>[2x]MAETPNSDMSGATGGRSKRPKSNQDWWPSKLNLEILDQNARDVGPVEDDFDYAEEFQKLDLEAVKSDLEEL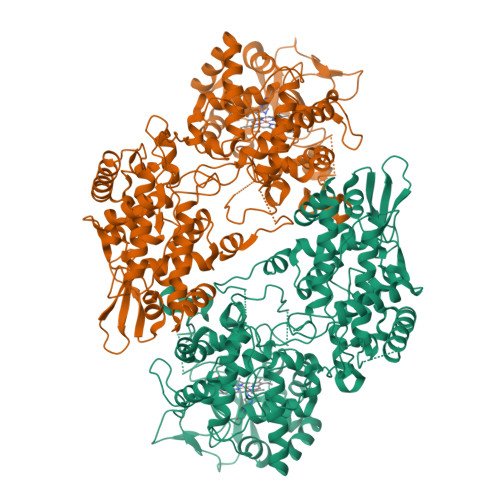MTSSQDWWPADYGHYGPLFIRMAWHSAGTYRTADGRGGAAGGRQRFAPINSWPDNANLDKARRLLLPIKQKYGQKISWADLMILAGNVAIESMGFKTFGYAGGREDAFEEDKAVNWGPEDEFETQERFDEPGEIQEGLGASVMGLIYVNPEGPDGNPDPEASAKNIRQTFDRAAMNDKETAALIAGGHTFGKVHGADDPEENLGPEPEAAPIEQQGLGWQNKNGNSKGGEMITSGIEGPWTQSPTEWDMGYINNLLDYEWEPEKGPGGAWQWAPKSEELKNSVPDAHDPDEKQTPMMLTTDIALKRDPDYREVMETFQENPMEFGMNFAKAWYKLTHRDMGPPERFLGPEVPDEEMIWQDPLPDADYDLIGDEEIAELKEEILDSDLSVSQLVKTAWASASTYRDSDKRGGANGARLRLEPQKNWEVNEPEQLETVLGTLENIQTEFNDSRSDGTQVSLADLIVLGGNAAVEQAAANAGYDVEIPFEPGRVDAGPEHTDAPSFDALKPKVDGVRNYIQDDITRPAEEVLVDNADLLNLTASELTALIGGMRSIGANYQDTDLGVFTDEPETLTNDFFVNLLDMGTEWEPAADSEHRYKGLDRDTGEVKWEATRIDLIFGSNDRLRAISEVYGSADAEKKLVHDFVDTWSKVMKLDRFDLEHHHHHH4-(3-PYRIDIN-2-YL-1H-PYRAZOL-4-YL)QUINOLINE 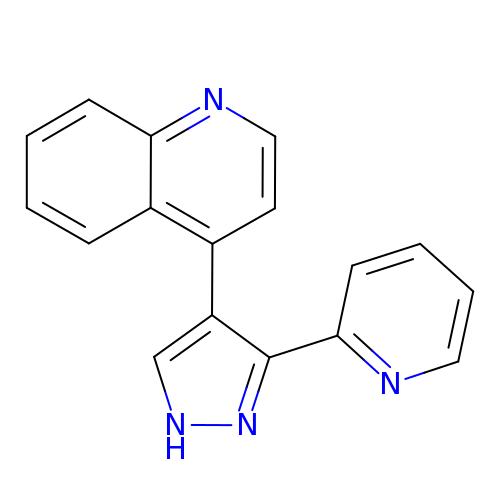| C17 H12 N4 | IBCXZJCWDGCXQT-UHFFFAOYSA-N> VLSQAQAQNSQYALARTFATQKVSLEE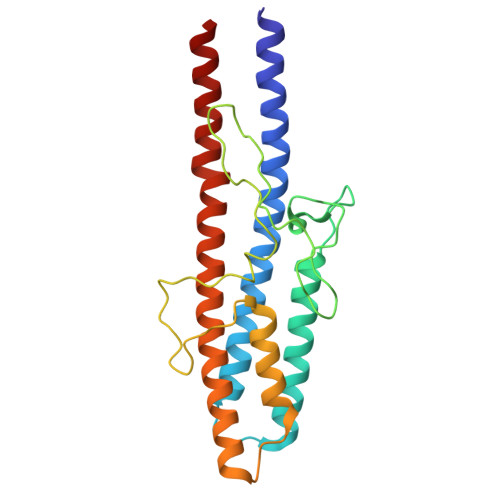SVLSQVTTAIQTAQEKIVYAGNGTLSDDDRASLATDLQGIRDQLMNLANSTDGNGRYIFAGYKTEAAPFDQATGGYHGGEKSVTQQVDSARTMVIGHTGAQIFNSITSNAVPEPDGSDSEKNLFVMLDTAIAALKTPVEGNNVEKEKAAAAIDKTNRGLKNSLNNVLTVRAELGTQLSELSTLDSLGSDRALGQKL>[4x]MSLTPLMVNGILGESVTLPLEFPAGEKVNFITWLFNETSLAFIVPHETKSPEIHVTNPKQGKRLNFTQSYSLQLSN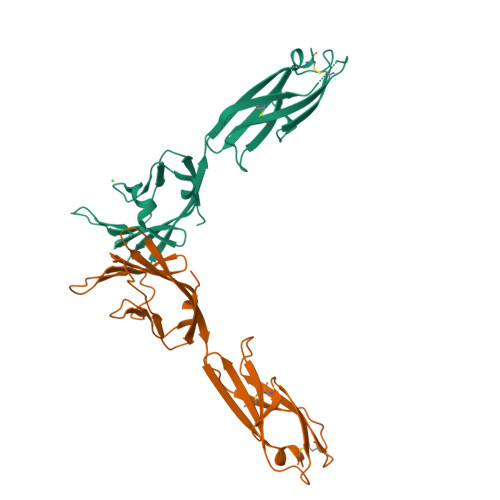LKMEDTGSYRAQISTKTSAKLSSYTLRILRQLRNIQVTNHSQLFQNMTCELHLTCSVEDADDNVSFRWEALGNTLSSQPNLTVSWDPRISSEQDYTCIAENAVSNLSFSVSAQKLCE(2R)-2-(cyclopentylmethyl)-N'-{5-fluoro-6-[(9aS)-hexahydropyrazino[2,1-c][1,4]oxazin-8(1H)-yl]-2-methylpyrimidin-4-yl}-3-[hydroxy(hydroxymethyl)amino]propanehydrazide 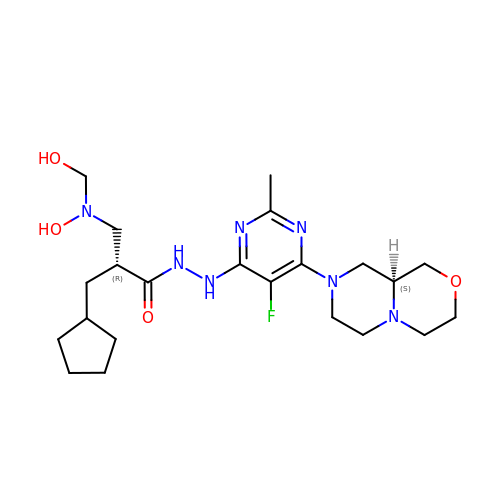| C22 H36 F N7 O4 | ZUQCOBLJLUYLKK-MSOLQXFVSA-N>[4x]GAMGSSGWCIFIYNLGQDA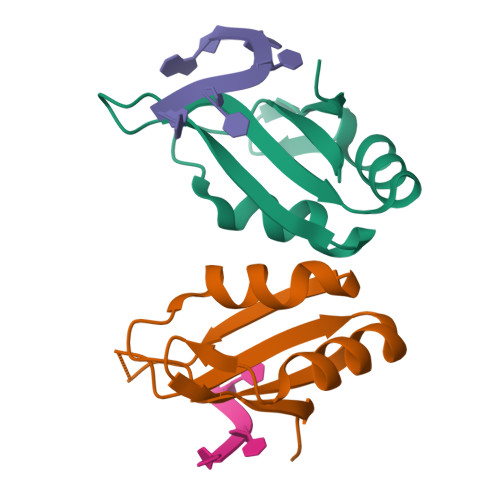DEGILWQMFGPFGAVTNVKVIRDFNTNKCKGFGFVTMTNYEEAAMAIASLNGYRLGDKILQVSFKTNKSHK> MLGTGPAAATTAATTSXXXXXXXXXXXXXXSRNEETXXXXXXXXXXXXXXXXXEMSQEEXTRFYDQLNHHIFELVSSSDANERKGGILAIASLIGVEGGNATRIGRFANYLRNLLPSNDPVVMEMASKAIGRLAMAGDTFTAEYVEFEVKRALEWLGADRNEGRRHAAVLVLRELAISVPTFFFQQVQPFFDNIFVAVWDPKQAIREGAVAALRACLILTTQREPKEMQKPQWYRHTFEEAEKGFDETLAKEKGMNRDDRIHGALLILNELVRISSMEGERLREEMEEITQQQLVHDKYCKDLMGFGTKPRHITPFTSFQAVQPQQSNALVGLLGYSSHQGLMGFGTSPSPAKSTXXXXXXXXXXXXXXXXXXXXXXXKCRNSKNSLIQMTILNLLPRLAAFRPSAFTDTQYLQDTMNHVLSCVKKEKERTAAFQALGLLSVAVRSEFKVYLPRVLDIIRAALPPKDFAHKRQKAMQVDATVFTCISMLARAMGPGIQQDIKELLEPMLAVGLSPALTAVLYDLSRQIPQLKKDIQDGLLKMLSLVLMHKPLRHPGMPKGLAHQLASPGLTTLPEASDVGSITLALRTLGSFEFEGHSLTQFVRHCADHFLNSEHKEIRMEAARTCSRLLTPSIHLISGHAHVVSQTAVQVVADVLSKLLVVGITDPDPDIRYCVLASLDERFDAHLAQAENLQALFVALNDQVFEIRELAICTVGRLSSMNPAFVMPFLRKMLIQILTELEHSGIGRIKEQSARMLGHLVSNAPRLIRPYMEPILKALILKLKDPDPDPNPGVINNVLATIGELAQVSGLEMRKWVDELFIIIMDMLQDSSLLAKRQVALWTLGQLVASTGYVVEPYRKYPTLLEVLLNFLKTEQNQGTRREAIRVLGLLGALDPYKHKVNIGMIDQSRDASAVSLSESKSSQDSSDYSTSEMLVNMGNLPLDEFYPAVSMVALMRIFRDQSLSHHHTMVVQAITFIFKSLGLKCVQFLPQVMPTFLNVIRVCDGAIREFLFQQLGMLVSFVKSHIRPYMDEIVTLMREFWVMNTSIQSTIILLIEQIVVALGGEFKLYLPQLIPHMLRVFMHDNSPGRIVSIKLLAAIQLFGANLDDYLHLLLPPIVKLFDAPEAPLPSRKAALETVDRLTESLDFTDYASRIIHPIVRTLDQSPELRSTAMDTLSSLVFQLGKKYQIFIPMVNKVLVRHRINHQRYDVLICRIVKGYTLADEEEDPLIYQHRMLRSGQGDALASGPVETGPMKKLHVSTINLQKAWGAARRVSKDDWLEWLRRLSLELLKDSSSPSLRSCWALAQAYNPMARDLFNAAFVSCWSELNEDQQDELIRSIELALTSQDIAEVTQTLLNLAEFMEHSDKGPLPLRDDNGIVLLGERAAKCRAYAKALHYKELEFQKGPTPAILESLISINNKLQQPEAAAGVLEYAMKHFGELEIQATWYEKLHEWEDPLVAYDKKMDTNKDDPELMLGRMRCLEALGEWGQLHQQCCEKWTLVNDETQAKMARMAAAAAWGLGQWDSMEEYTCMIPRDTHDGAFYRAVLALHQDLFSLAQQCIDKARDLLDAELTAMAGESYSRAYGAMVSCHMLSELEEVIQYKLVPERREIIRQIWWERLQGCQRIVEDWQKILMVRSLVVSPHEDMRTWLKYASLCGKSGRLALAHKTLVLLLGVDPSRQLDHPLPTVHPQVTYAYMKNMWKSARKIDAFQHMQHFVQTMQQQAQHAIATEDQQHKQELHKLMARCFLKLGEWQLNLQGINESTIPKVLQYYSAATEHDRSWYKAWHAWAVMNFEAVLHYKHQNQARDEKKKLRHASGANITNATTAATTAATATTTASTEGSNSESEAESTENSPTPSPLQKKVTEDLSKTLLMYTVPAVQGFFRSISLSRGNNLQDTLRVLTLWFDYGHWPDVNEALVEGVKAIQIDTWLQVIPQLIARIDTPRPLVGRLIHQLLTDIGRYHPQALIYPLTVASKSTTTARHNAANKILKNMCEHSNTLVQQAMMVSEELIRVAILWHEMWHEGLEEASRLYFGERNVKGMFEVLEPLHAMMERGPQTLKETSFNQAYGRDLMEAQEWCRKYMKSGNVKDLTQAWDLYYHVFRRISKQLPQLTSLELQYVSPKLLMCRDLELAVPGTYDPNQPIIRIQSIAPSLQVITSKQRPRKLTLMGSNGHEFVFLLKGHEDLRQDERVMQLFGLVNTLLANDPTSLRKNLSIQRYAVIPLSTNSGLIGWVPHCDTLHALIRDYREKKKILLNIEHRIMLRMAPDYDHLTLMQKVEVFEHAVNNTAGDDLAKLLWLKSPSSEVWFDRRTNYTRSLAVMSMVGYILGLGDRHPSNLMLDRLSGKILHIDFGDCFEVAMTREKFPEKIPFRLTRMLTNAMEVTGLDGNYRITCHTVMEVLREHKDSVMAVLEAFVYDPLLNWRLMDTNTKGNKRSRTRTDSYSAGQSVEILDGVELGEPAHKKTGTTVPESIHSFIGDGLVKPEALNKKAIQIINRVRDKLTGRDFSHDDTLDVPTQVELLIKQATSHENLCQCYIGWCPFW;> MNTSPGTVGSDPVILATAGYDHTVRFWQAHSGICTRTVQHQDSQVNALEVTPDRSMIAAAGYQHIRMYDLNSNNPNPIISYDGVNKNIASVGFHEDGRWMYTGGEDCTARIWDLRSRNLQCQRIFQVNAPINCVCLHPNQAELIVGDQSGAIHIWDLKTDHNEQLIPEPEVSITSAHIDPDASYMAAVNSTGNCYVWNLTGGIGDEVTQLIPKTKIPAHTRYALQCRFSPDSTLLATCSADQTCKIWRTSNFSLMTELSIKSGNPGESSRGWMWGCAFSGDSQYIVTASSDNLARLWCVETGEIKREYGGHQKAVVCLAFNDSVLG;> MEEGGSTGSAGSDSSTSGSGGAQQRELERMAEVLVTGEQLRLRLHEEKVIKDRRHHLKTYPNCFVAKELIDWLIEHKEASDRETAIKLMQKLADRGIIHHVCDEHKEFKDVKLFYRFRKDDGTFPLDNEVKAFMRGQRLYEKLMSPENTLLQPREEEGVKYERTFMASEFLDWLVQEGEATTRKEAEQLCHRLMEHGIIQHVSSKHPFVDSNLLYQFRMNFRRRRRLMELLNEKSPSSQETHDSPFCLRKQSHDNRKSTSFMSVSPSKEIKIVSAVRRSSMSSCGSSGYFSSSPTLSSSPPVLCNPKSVLKRPVTSEELLTPGAPYAR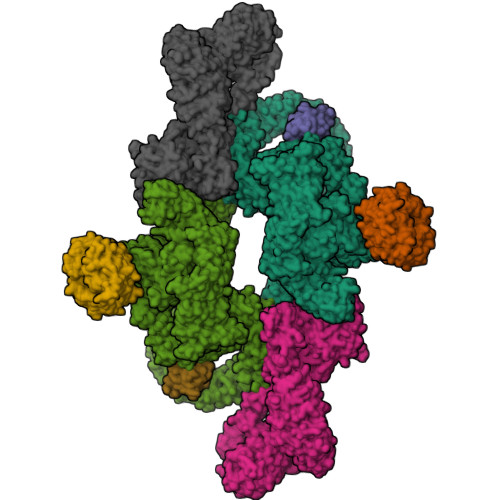KTFTIVGDAVGWGFVVRGSKPCHIQAVDPSGPAAAAGMKVCQFVVSVNGLNVLHVDYRTVNNLILTGPRTIVMEVMEELEC;> MESEMLQSPLLGLGEEDEADLTDWNLPLAFMKKRHCEKIEGSKSLAQSWRMKDRMKTVSVALVLCLNVGVDPPDVVKTTPCARLECWIDPLSMGPQKALETIGANLQKQYENWQPRARYKQSLDPTVDEVKKLCTSLRRNAKEERVLFHYNGHGVPRPTVNGEVWVFNKNYTQYIPLSIYDLQTWMGSPSIFVYDCSNAGLIVKSFKQFALQREQELEVAAINPNHPLAQMPLPPSMKNCIQLAACEATELLPMIPDLPADLFTSCLTTPIKIALRWFCMQKCVSLVPGVTLDLIEKIPGRLNDRRTPLGELNWIFTAITDTIAWNVLPRDLFQKLFRQDLLVASLFRNFLLAERIMRSYNCTPVSSPRLPPTYMHAMWQAWDLAVDICLSQLPTIIEEGTAFRHSPFFAEQLTAFQVWLTMGVENRNPPEQLPIVLQVLLSQVHRLRALDLLGRFLDLGPWAVSLALSVGIFPYVLKLLQSSARELRPLLVFIWAKILAVDSSCQADLVKDNGHKYFLSVLADPYMPAEHRTMTAFILAVIVNSYHTGQEACLQGNLIAICLEQLNDPHPLLRQWVAICLGRIWQNFDSARWCGVRDSAHEKLYSLLSDPIPEVRCAAVFALGTFVGNSAERTDHSTTIDHNVAMMLAQLVSDGSPMVRKELVVALSHLVVQYESNFCTVALQFIEEEKNYALPSPATTEGGSLTPVRDSPCTPRLRSVSSYGNIRAVATARSLNKSLQNLSLTEESGGAVAFSPGNLSTSSSASSTLGSPENEEHILSFETIDKMRRASSYSSLNSLIGVSFNSVYTQIWRVLLHLAADPYPEVSDVAMKVLNSIAYKATVNARPQRVLDTSSLTQSAPASPTNKGVHIHQAGGSPPASSTSSSSLTNDVAKQPVSRDLPSGRPGTTGPAGAQYTPHSHQFPRTRKMFDKGPEQTADDADDAAGHKSFISATVQTGFCDWSARYFAQPVMKIPEEHDLESQIRKEREWRFLRNSRVRRQAQQVIQKGITRLDDQIFLNRNPGVPSVVKFHPFTPCIAVADKDSICFWDWEKGEKLDYFHNGNPRYTRVTAMEYLNGQDCSLLLTATDDGAIRVWKNFADLEKNPEMVTAWQGLSDMLPTTRGAGMVVDWEQETGLLMSSGDVRIVRIWDTDREMKVQDIPTGADSCVTSLSCDSHRSLIVAGLGDGSIRVYDRRMALSECRVMTYREHTAWVVKASLQKRPDGHIVSVSVNGDVRIFDPRMPESVNVLQIVKGLTALDIHPQADLIACGSVNQFTAIYNSSGELINNIKYYDGFMGQRVGAISCLAFHPHWPHLAVGSNDYYISVYSVEKRVR>[12x]HGTELIKRGFARMQKGGVIMDVTTPEQARIAEEAGAVAVMALQAVPADIRKAGGVARMADPEIVQQIIETVTIPVMAKARIGHFVEAEILEALGVDMVDESEVLTPADPFYHIDKTQFTVPFVCGARNLGEALRRINEGAAMIRTKGEAGTGDVSQAVKHMKQIQGEIRALAGKTKEELIMVAREIEAPIELVVETAKMQRLPVVNFAAGGVATPADAALMMRLGADGVFVGSGIFKAENPEKMAKAVVEAVNNYDNPVKLAEISKGVGAGMKGISADMIPAQEALQERGW

Through the cryoID approach, we successfully reconstructed and identified the native Methanosarcina acetivorans pyridoxal 5′-phosphate (PLP) synthase (PdxS) complex directly from cryogenic electron microscopy (cryo-EM) images of fractionated cellular lysate. PLP is the biologically active state of vitamin B6, participating in over 160 crucial enzymatic processes, which include the metabolism of glycogen, amino acids, and lipids. Each monomer adapts a triose phosphate isomerase (TIM) barrel fold that houses the active site for deoxyxylulose 5-phosphate-independent PLP synthesis from D-ribose 5-phosphate (R5P), D-glyceraldehyde 3-phosphate, and an ammonia moiety from glutamine. Like other homologous PLP synthase structures, the M. acetivorans PdxS dodecameric complex consists of two layers of homohexameric rings that stack cylindrically, with an outer diameter of 108 Å and an inner diameter of 42 Å.

Similar classes were noted between negative stain and cryo-EM 2D averaging, and by employing a single-particle analysis approach with the cryoSPARC suite, we reconstructed a cryo-EM map to 3.38 Å with D6 symmetry. We found that the native PdxS complex exists as a homo-dodecamer of PdxS subunits, and the previously proposed supracomplex containing both the synthase (PdxS) and glutaminase (PdxT) was not observed in cellular lysate. Our structure shows that the native PdxS monomer fashions a single 8α/8β TIM-barrel domain, surrounded by seven additional helices to mediate solvent and interface contacts. Monomer tips also interdigitate at the hexamer-hexamer interface, creating altogether three distinct types of lateral contacts that give rise to the dodecamer, here described as AB, AA, and BB. A network of six inter-subunit hydrogen bonds anneal the facets of interface AB together, while two such interactions comprise AA, and another four comprise BB (while each has 1 and 2 unique bonds, respectively, these are doubled due to the inherent twofold symmetry of the “self” interfaces). The first 10 residues lack clear density for modeling, as was similarly observed with the Arabidopsis thaliana Pdx1.2/1.3 pseudoenzyme structures, indicating that this region is relatively flexible when unbound to its glutaminase, PdxT. The M. acetivorans αN helix displays several solvent-exposed hydrophobic residues (I16, G19, F20, M23), with regions of dense negative and positive charge above and below, respectively, which is highly suggestive of a putative binding interface for the glutaminase. In our maps, no instances of PdxT binding were observed, even after extensive 3D classification and examination under a low-density threshold. Based on comparison with previous crystal structures where PdxS was co-crystallized with R5P and various intermediate states, the density is most likely to belong to either bound R5P or an R5P Schiff-base intermediate.> AMGKLLTMAMPKGRIFEEAAGLLRQAGYRLPEEFEDSRKLIIDVPEENLRFILAKPMDVTTYVEHGVA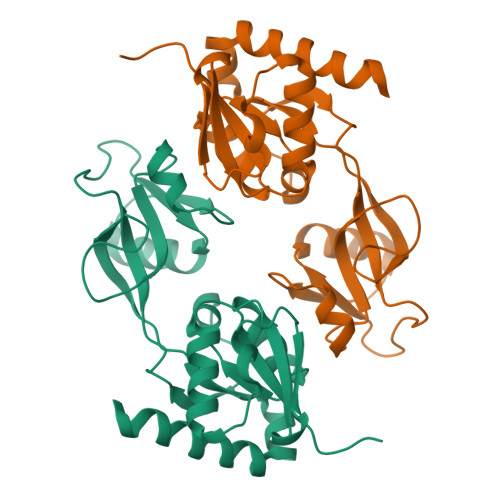DVGIAGKDVMLEEERDVYEVLDLNISKCHLAVAGLPNTDWSGVAPRIATKYPNVASSYFREQGEQVEIIKLNGSIELAPLIGLADRIVDIVSTGQTLKENGLVETEHICDITSRFIVNPVSYRMKDDVIDEMASRLSLVVEGETAK> EDSLGMEVGYRLIPMVDFQQDGELLGRIRSIRKKFAQDMGFLPPVVHIRDNMDLQPARYRILMKGVEIGSGDAYPGRWLAINPGTAAGTLPGEKTVDPAFGLDAIWIESALKEQAQIQGFTVVEA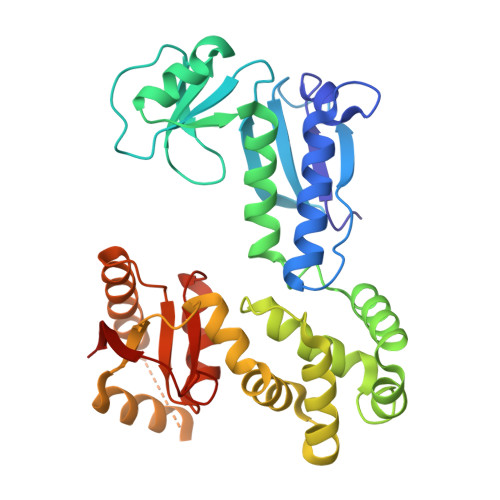STVVATHLNHLIGQFSAELFGRQEAQQLLDRVSQEMPKLTEDLVPGVVTLTTLHKVLQNLLAEKVPIRDMRTILETLAEHAPLQSDPHELTAVVRVALGRAITQQWFPGNEEVQVIGLDTALERLLLQALQGGGGLEPGLADRLLAQTQEALSRQEMLGAPPVLLVNHALRPLLSRFLRRSLPQLVVLSNLELSDNRHIRMTATIG> MGSSLRPLYMDVQATTPLDPRVLDAMLPYLINYYGNPHSRTHAYGWESEAAMERARQQVASLIGADPREIIFTSGATESNNIAIKGVARFYRSRKKHLITTQTEHKCVLDSCRSLEAEGFQVTYLPVQKSGIIDLKELEAAIQPDTSLVSVMTVNNEIGVKQPIAEIGRICSSRKVYFHTDAAQAVGKIPLDVNDMKIDLMSISGHKIYGPKGVGAIYIRRRPRVRVEALQSGGGQERGMRSGTVPTPLVVGLGAACEVAQQEMEYDHKRISKLSERLIQNIMKSLPDVVMNGDPKHHYPGCINLSFAYVEGESLLMALKDVALSSGSACTSASLEPSYVLRAIGTDEDLAHSSIRFGIGRFTTEEEVDYTVEKCIQHVKRLREMSPLWEMVQDGIDLKSIKW;> MAASSRAQVLALYRAMLRESKRFSAYNYRTYAVRRIRDAFRENKNVKDPVEIQTLVNKAKRDLGVIRRQVHIGQLYSTDKLIIENRDMPRT;> STIEERVKKIIGEQLGVKQEEVTNNASFVEDLGADSLDTVELVMALEEEFDTEIPDEEAEKITTVQAAIDYINGHQ;> MAYHKKVVDHYENPRNVGSLDKTSKNVGTGLVGAPACGDVMKLQIQVDEKGKIVDARFKTFGCGSAIASSSLATEWVKGKTVEEALTIKNTDIAKELCLPPVKLHCSMLAEDAIKAALADYKLKQEPKKGEAEKK

Intracellular d-Cys specifically inhibits the mitochondrial cysteine desulfurase NFS1, a key enzyme of cellular iron–sulfur protein biogenesis, by blocking sulfur mobilization due to steric constraints. Because NFS1 catalyses the sulfur release from l-Cys producing alanine and a persulfide (-SSH) on its active-site residue Cys381, the enzyme is a likely target of d-Cys. Briefly, the reaction cycle of the pyridoxal phosphate (PLP)-dependent NFS1 (and related desulfurases) involves the conversion of the Lys258NFS1-bound internal aldimine (that is, an NFS1-bound PLP via Schiff base formation) to external (that is, non-protein-bound) Cys-aldimine and Cys-ketimine followed by generation of Ala-ketimine and concomitant Cys sulfur release for persulfide formation on Cys381NFS1.

However, in the NFS1 active site, we observed an external l-propargylglycine-ketimine, which is an analogue of the external Cys-ketimine intermediate that can be formed by both l-Cys and d-Cys. This l-propargylglycine-ketimine was structurally similar to a l-propargylglycine bound to the class II cysteine desulfurase SufS from Bacillus subtilis. Therefore, we used our structure to model either an l-Cys-ketimine or a d-Cys-ketimine into the active centre of NFS1. In creating these models, we superimposed the N-Cα-C(O) backbone of l-Cys or d-Cys on that of l-propargylglycine. In the case of l-Cys-ketimine, the Cys sulfur was located in close proximity to both the strictly conserved proton-abstracting His156NFS1 (2.9 Å)46 and the persulfide-accepting Cys381NFS1 (2.8 Å). In our NFS1 model, the d-Cys-ketimine sulfur was positioned in the almost opposite direction compared with l-Cys-ketimine, pointing towards Lys258NFS1. As a consequence, the sulfur was located far from both His156NFS1 and Cys381NFS1 (3.6 Å and 5.4 Å, respectively), thus making sulfur transfer to Cys381NFS1 both catalytically and sterically unfavourable. We conclude that the altered location of the d-Cys sulfur is incompatible with sulfur mobilization and persulfidation. In summary, NFS1 readily and efficiently forms the Cys-ketimine intermediate with both l-Cys and d-Cys but steric hindrance in the case of d-Cys prevents subsequent sulfur transfer to the acceptor Cys381NFS1.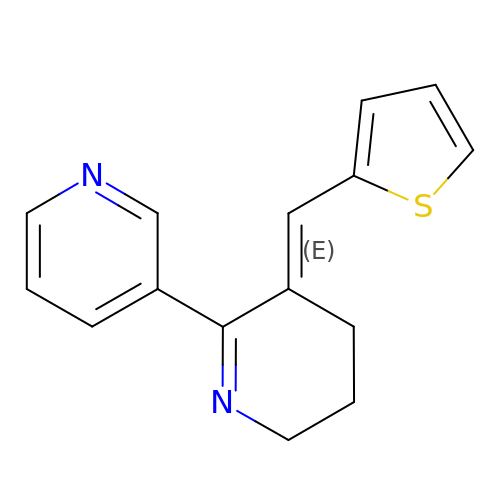(3E)-3-(thiophen-2-ylmethylidene)-3,4,5,6-tetrahydro-2,3'-bipyridine | C15 H14 N2 S | MYYXDAYQWWIEQW-ZRDIBKRKSA-N>ASAKLPGDFGPPRGEPIHAVLTSPPLVPPPVNRTYPAK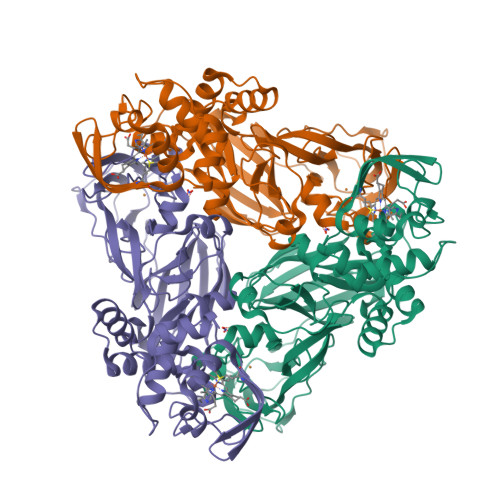VIVELEVVEKEMQISEGVSYTFWTFGGTVPGSFIRVRQGDTVEFHLKNHPSSKMPHNIDLHGVTGPGGGAASSFTAPGHESQFTFKALNEGIYVYHCATAPVGMHIANGMYGLILVEPPEGLPKVDHEYYVMQGDFYTAGKYREKGLQPFDMEKAIDERPSYVLFNGAEGALTGDKALHAKVGETVRIFVGNGGPNLVSSFHVIGAIFDQVRYEGGTNVQKNVQTTLIPAGGAAVVKFTARVPGSYVLVDHSIFRAFNKGAMAILKIDGAENKLVYSGKELDSVALGDRAAPNMSAVTKATQASVSGTLTVQDQVQAGRALFAGTCSVCHQGNGAGLPGVFPPLAKSDFLAADPKRAMNIVLHGLNGKIKVNGQEYDSVMPPMTQLNDDEVANILTYVLNSWDNPGGRVSAEDVKKVRAQPAPAKAVAEH[2x]4-[({3-HYDROXY-2-METHYL-5-[(PHOSPHONOOXY)METHYL]PYRIDIN-4-YL}METHYL)AMINO]THIOPHENE-2-CARBOXYLIC 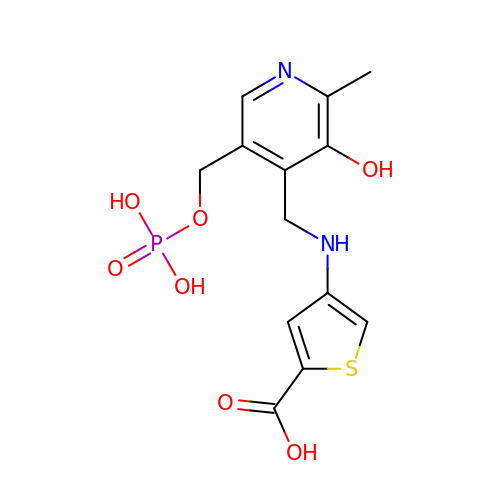ACID | C13 H15 N2 O7 P S | SUKBSASAEROGCJ-UHFFFAOYSA-N> MNDRADFVVPDITTRKNVGLSHDANDFTLPQPLDRYSAEDHATWATLYQRQCKLLPGRACDEFLEGLERLEVDADRVPDFNKLNEKLMAATGWKIVAVPGLIPDDVFFEHLANRRFPVTWWLREPHQLDYLQEPDVFHNLFG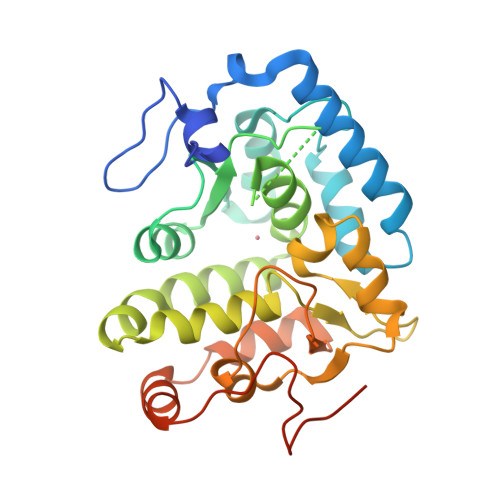HVPLLINPVFADYLEAYGKGGVKAKALGALPMLARLYWYTVEFGLINTPAGMRIYGAGILSSKSESIYCLDSASPNRVGFDLMRIMNTRYRIDTFQKTYFVIDSFKQLFDATAPDFAPLYLQLADAQPWGAGDIAPDDLVLNAGDRQGWADTEDV> MSGKLRLYKEKLEGYNRFYSIVKTIKMVTLAKYRAAQGRIRTRDFSLRYTELAFSKPQASRDAVVAAKNALVYIPITTNRGSCGALNSNIVRCIDSVVSSKMVLMPVGKRGIDSFSKLYPDEFRYGIINDMKESMHFGYATF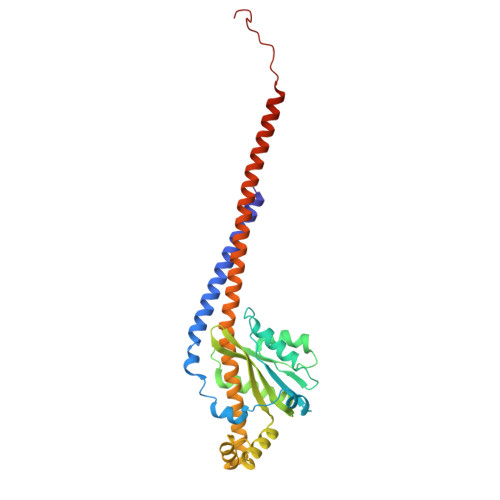VIENAYEVSKDADRYQVIFNRFVSAGVQRNAVYNIPSYEKWKEDLADAASSDNQKNRYLFANALQNEEEQLIRDFFDFHAALAVLNAVGENELSEQAARLVAVEGQLTNISSLQQRTSSLYNKTRQFGITAALIEILSAMSSLEGNAMKGVRRNKFWEGAVTK> MKYFTVFTALTALFAQASASAIPAVRSTLTPRQNTTASCANSATSRSCWGEYSIDTNWYDVTPTGVTREYWLSVENSTITPDGYTRSAMTFNGTVPGPAIIADWGDNLIIHVTNNLEHNGTSIHWHGIRQLGSLEYDGVPGVTQCPIAPGDTLTYKFQV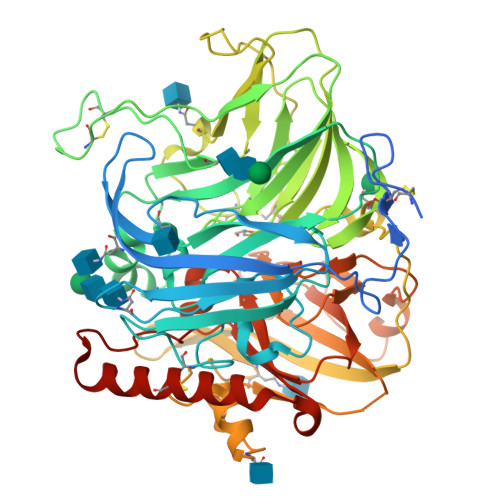TQYGTTWYHSHFSLQYGDGLFGPLIINGPATADYDEDVGVIFLQDWAHESVFEIWDTARLGAPPALENTLMNGTNTFDCSASTDPNCVGGGKKFELTFVEGTKYRLRLINVGIDSHFEFAIDNHTLTVIANDLVPIVPYTTDTLLIGIGQRYDVIVEANAAADNYWIRGNWGTTCSTNNEAANATGILRYDSSSIANPTSVGTTPRGTCEDEPVASLVPHLALDVGGYSLVDEQVSSAFTNYFTWTINSSSLLLDWSSPTTLKIFNNETIFPTEYNVVALEQTNANEEWVVYVIEDLTGFGIWHPIHLHGHDFFIVAQETDVFNSDESPAKFNLVNPPRRDVAALPGNGYLAIAFKLDNPGSWLLHCHIAWHASEGMAMQFVESQSSIAVKMTDTAIFEDTCANWNAYTPTQLFAEDDSGI3-[3-(2-acetamidoethyl)phenyl]benzoic acid | 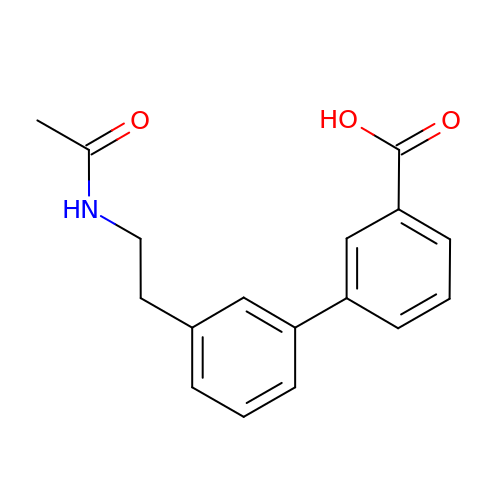C17 H17 N O3 | VSVONDXWDQOLJS-UHFFFAOYSA-N> SSTGSI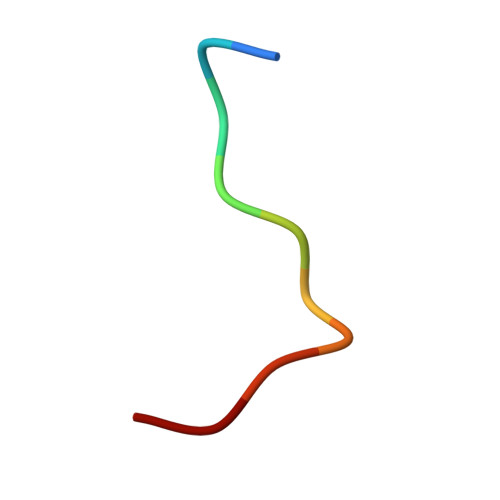DMVD D-MONAPTERIN 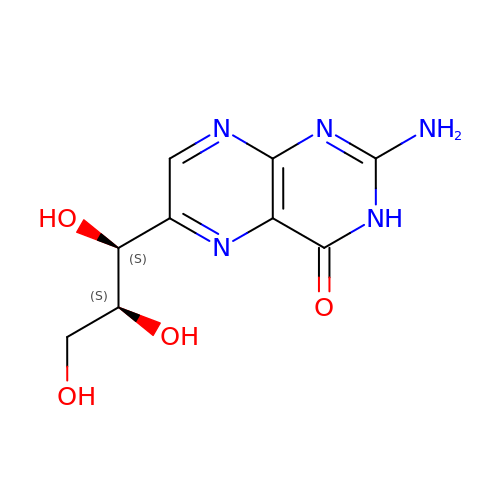| C9 H11 N5 O4 | BMQYVXCPAOLZOK-NJGYIYPDSA-N>[2x]ALLKFDLFYGRTDAQIKSLLDAAHGAMVDAFGVPANDRYQTVSQHRPGE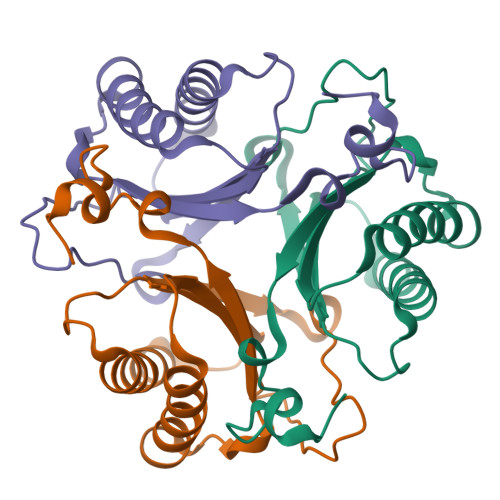MVLEDTGLGYGRSSAVVLLTVISRPRSESQKVCFYKLLTGALERDCGISPDDVIVALVENSDADWSFGRGRAEFLTGDLVG(2R,3R,4R)-3,4-dihydroxy-5-oxooxan-2-yl [(2R,3S,4R,5R)-5-(2,4-dioxo-3,4-dihydropyrimidin-1(2H)-yl)-3,4-dihydroxyoxolan-2-yl]methyl dihydrogen 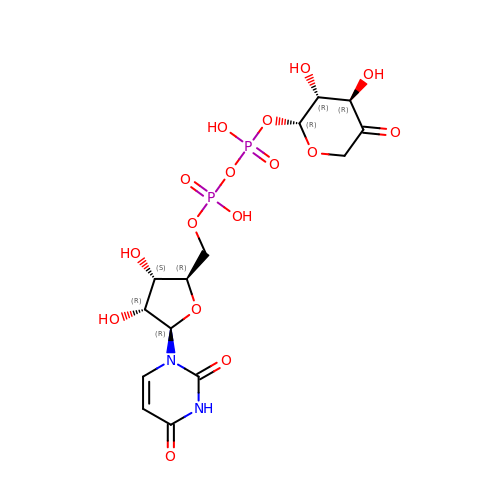diphosphate (non-preferred name) | C14 H20 N2 O16 P2 | URJZIQLTPCJVMW-QNSCKLTRSA-N> 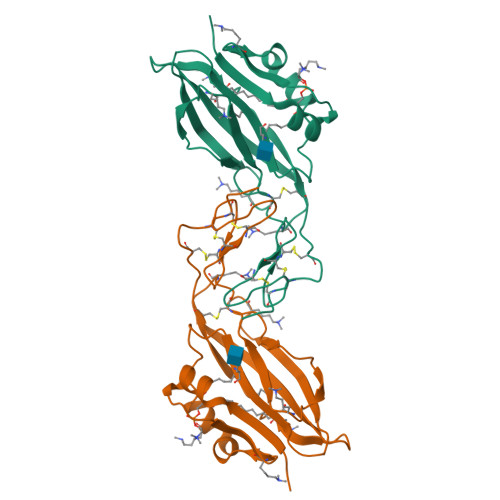ETGSLYLWIDAHQARVLIGFEEDILIVSEGKMAPFTHDFRKAQQRMPAIPVNIHSMNFTWQAAGQAEYFYEFLSLRSLDKGIMADPTVNVPLLGTVPHKASVVQVGFPCLGKQDGVAAFEVDVIVMNSEGNTILKTPQNAIFFKTCQQAECPGGCRNGGFCNERRICECPDGFHGPHCEGTKHHHHHH>TDTFQMFWLDYCEVNNTLILFGKVKLKDDNCVSAMVQINGLCRELFFLPREGKTPTDIHEEIIPLLMDKYGLDNIRAKPQKMKYSFELPDIPSESDYLKVLLPYQTPKSSRDTIPSDLSSDTFYHVFGGNSNIFESFVIQNRIMGPCWLDIKGADFNSIRNASHCAVEVSVDKPQNITPTTTKTMPNLRCLSLSIQTLMNPKENKQEIVSITLSAYRNISLDSPIPENIKPDDLCTLVRPPQSTSFPLGLAALAKQKLPGRVRLFNNEKAMLSCFCAMLKVEDPDVIIGHRLQNVYLDVLAHRMHDLNIPTFSSIGRRLRRTWPEKFGRGNSNMNHFFISDICSGRLICDIANEMGQSLTPKCQSWDLSEMYQVTCEKEHKPLDIDYQNPQYQNDVNSMTMALQENITNCMISAEVSYRIQLLTLTKQLTNLAGNAWAQTLGGTRAGRNEYILLHEFSRNGFIVPDKEGNRSRAQKQRQNEENADAPVNSKKAKYQGGLVFEPEKGLHKNYVLVMDFNSLYPSIIQEFNICFTTVDRNKEDIDELPSVPPSEVDQGVLPRLLANLVDRRREVKKVMKTETDPHKRVQCDIRQQALKLTANSMYGCLGYVNSRFYAKPLAMLVTNKGREILMNTRQLAESMNLLVVYGDTDSVMIDTGCDNYADAIK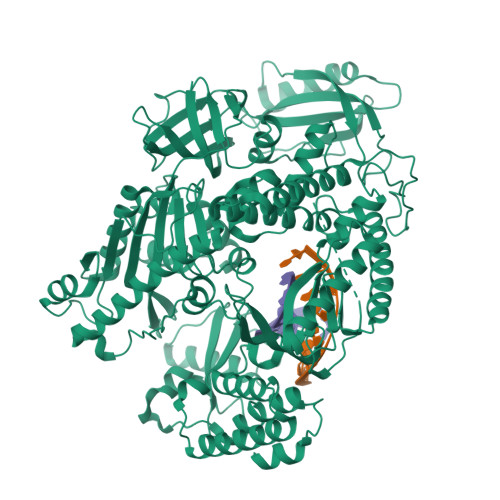IGLGFKRLVNERYRLLEIDIDNVFKKLLLHAKKKYAALTVNLDKNGNGTTVLEVKGLDMKRREFCPLSRDVSIHVLNTILSDKDPEEALQEVYDYLEDIRIKVETNNIRIDKYKINMKLSKDPKAYPGGKNMPAVQVALRMRKAGRVVKAGSVITFVITKQDEIDNAADTPALSVAERAHALNEVMIKSNNLIPDPQYYLEKQIFAPVERLLERIDSFNVVRLSEALGLDSKKYFRREGGNNNG[2x]> GPNLDFQALEETTEYDGGYTRDSVLIR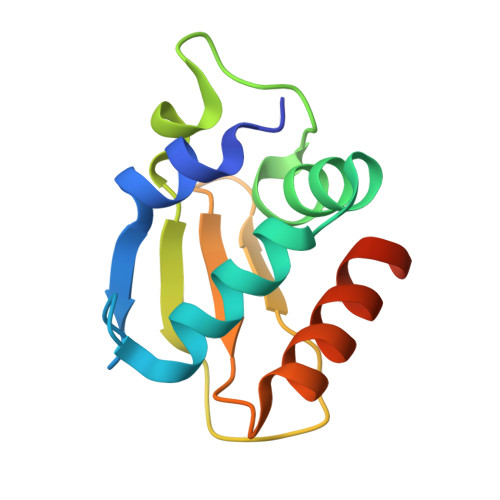EFWEIVHSFTDEQKRLFLQFTTGTDRAPVGGLGKLKMIIAKNGPDTERLPTSHTCFNVLLLPEYSSKEKLKERLLKAITYAKGFGML Myophage Mu is a representative of contractile nanomachines with a simple tail baseplate. It has the capacity to infect a range of intestinal bacteria and has extensive applications in genetic engineering research. Using cryo-EM, we resolved the three-dimensional (3D) structures of the G(+) type phage Mu in both its extended state and urea-induced contracted state, the latter lacking the baseplate, at near-atomic resolutions. The structure of extended Mu can be divided into four distinct regions: the DNA-containing head, the connector complex, the tail, and the baseplate.

By employing the symmetry mismatch reconstruction and the local reconstruction methods, the structures of the portal-adaptor and the terminator-tail region of extended Mu were resolved to resolutions of 3.4 Å and 3.5 Å, respectively. The Mu tail terminator protein is constituted by six copies of protein gp37, and the tail sheath and tail tube of Mu are capped by the tail terminator, resulting in the termination of the assembly of the tail. The tail of Mu is comprised of 30 stacked hexameric tail protein rings, with the inner ring consisting of tube protein gp40 and the outer ring comprising sheath protein gp39. The tail tube protein gp40 adopts a conserved β-sandwich structural fold, exhibiting topological identity to that observed in myophages and CISs. Six copies of gp40 oligomerize to form a continuous 24-stranded β-barrel hexamer, with a β-hairpin of each gp40 protruding toward the adjacent ring to mediate the inter-ring interaction, which results in the formation of an extended helix tube structure with a helical rise of ~35 Å and a twist of ~25°. In addition, the inner surface of the tube exhibits a remarkably negative charge, which facilitates the passage of the DNA along the tube lumen. The tail sheath protein gp39 can be divided into five domains: N-arm, domain I, domain II, domain III, and C-arm. Domain I is responsible for the formation of the sheath inner wall, where an α-helix of the domain I in one tail sheath protein gp39 forms intermolecular contact with one inner tail tube protein gp40. Notably, the N-arm of one gp39 monomer and the C-arm of the adjacent monomer from the same sheath ring, together with a two-stranded β-sheet of the domain I from the adjacent sheath ring, form a “handshake” interaction by four-stranded β-sheet across two sheath rings, with the exception of the first and last layers of sheath ring. The domain I of the first layer of the sheath ring is linked to the BW1 gp46 (described below), and the domain I of the last layer interacts with the C-terminal β-hairpin domain of gp37 via the formation of an interlaced four-stranded β-sheet.

>MLEETEAALLARVRELFGATLRQVEPLTGTWTNEDVHRLFLAPPSVFLAWMGCGEGRTRREVESRWAFFVVAELLNGEPVNRPGIYQIVERLIAGVNGQTFGPTTGMRLTQVRNLCDDNRINAGVVLYGVLFSGTTPLPSVVDLDSLDDYERHWQTWKFPDETPEFAAHINVNQEKDHDAEN[6x];>MAGNQRQGVAFIRVNGMELESMEGASFTPSGITREEVTGSRVYGWKGKPRAAKVECKIPGGGPIGLDEIIDWENITVEFQADTGETWMLANAWQADEPKNDGGEISLVLMAKQSKRIA[12x];>[12x]MSDISFNAIPSDVRVPLTYIEFDNSNAVSGTPAPRQRVLMFGQSGSKASAAPNVPVRIRSGSQASAAFGQGSMLALMADAFLNANRVAELWCIPQGNGTGNAAVGEISLSGTAGENGSLVTYIAGQRLAVSVAAGATGAALADLLVARIKGQPDLPVTAEVRADSGDDDTHADVVLSAKFTGALSAVDVRWNYYAGETTPYGIITAFKAASGKNGNPDISASIAGMGDLQYKYIVMPYTDEPNLNLLRTELQERWGPVNQADGFAVTVLSGTYGDISTFGVSRNDHLISCMGIAGAPEPSYLYAATLCAVASQALSIDPARPLQTLTLPGRMPPAVGDRFTWSERNALLFDGISTFNVNDGGEMQIERMITMYRTNKYGDSDPSYLNVNTIATLSYLRYSLRTRITQKFPNYKLASDGTRFATGQAVVTPSVIKTELLALFEEWENAGLVEDFDTFKEELYVARNKDDKDRLDVLCGPNLINQFRIFAAQVQFIL> MGRLAIVVVATLALAAAAPPGKPSLGWGERTFAIVEVNQAATAYNQLVTKRDSADVSVTWNVWSGDPADKARVLLNDKEFWSGTGGAAGSASFKVKKGGRYQMVVELCNADGCSQSDATEIIVADTDGSHLPPLDYNMGEKNKPFKQTSGKVVG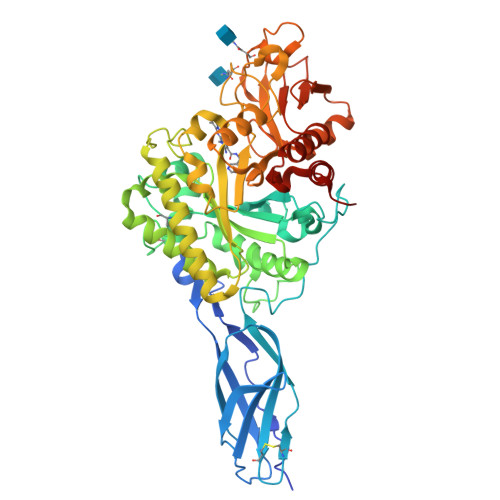AYFVEWGVYPRKFPVDRVPIPNLTHLLYGFIPICGGDGINDSLKEIEGSFQALQRSCSGREDFKVSIHDPWAALQKPQKGLSSWNEPYKGNFGQLMMLKQAKPDLKILPSIGGWTLADPFFFFTDETKRRRFVASVKDFLQTWKFFDGVDIDWEFPGGKGANPNLGSPKDGEIYVLLMKELREMLNELSAETGRKYELTSAISAGWDKIQVVDYSAAQKYMDHIFFMSYDFKGAWSNDTLGHQASLYAPDWNEKETYTTDFGVQFLLAQGVSPKKIVVGVAMYGRGWTGVHGYKDNNPFTGNATGPVKGTWQDGVVDYREIATEIAQGKWEYHYDKVAQAPYVFRPATGDLITYDDARSTIEKGKYVRANKLGGLFAWEIDADNGDILNAMNMGLGNSA>[2x]APDTSVSNKQNFSTDVIYQIFTDRFSDGNPANNPTGAAFDGSCTNLRLYCGGDWQGIINKINDGYLTGMGITAIWISQPVENIYSVINYSGVNNTAYHGYWARDFKKTNPAYGTMQDFKNLIDTAHAHNIKVIIDFAPNHTSPASSDDPSFAENGRLYDNGNLLGGYTNDTQNLFHHYGGTDLSTIENGIYKNLYDLADLNHN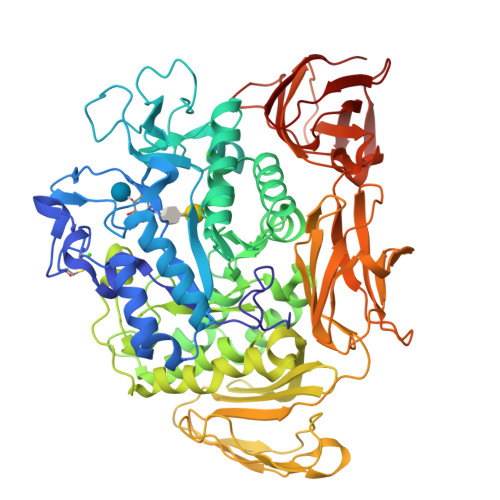NSSVDVYLKDAIKMWLDLGVDGIRVDAVKHMPFGWQKSFMATINNYKPVFTFGEWLLGVNEISPEYHQFANESGMSLLDFRFAQKARQVFRDNTDNMYGLKAMLEGSEVDYAQVNDQVTFIDNHDMERFHTSNGDRRKLEQALAFTLTSRGVPAIYYGSEQYMSGGNDPDNRARLPSFSTTTTAYQVIQKLAPLRKSNPAIAYGSTHERWINNDVIIYERKFGNNVAVVAINRNMNTPASITGLVTSLPRGSYNDVLGGILNGNTLTVGAGGAASNFTLAPGGTAVWQYTTDATTPIIGNVGPMMAKPGVTITIDGRGFGSGKGTVYFGTTAVTGADIVAWEDTQIQVKIPAVPGGIYDIRVANAAGAASNIYDNFEVLTGDQVTVRFVINNATTALGQNVFLTGNVSELGNWDPNNAIGPMYNQVVYQYPTWYYDVSVPAGQTIEFKFLKKQGSTVTWEGGANRTFTTPTSGTATVNVNWQP>MADKLFINALKKKFEESPEEKKTTFYTLGGWKQSERKTEFVNAGKEVAAKRGIPQYNPDIGTPLGQRVLMPYQVSTTDTYVEGDDLHFVNNAAMQQMWDDIRRTVIVGLNHAHAVIEKRLGKEVTPETITHYLETVNHAMPGAAVVQEHMVETHPALVADSYVKVFTGNDEIADEIDPAFVIDINKQFPEDQAETLKAEVGDGIWQVVRIPTIVSRTCDGATTSRWSAMQIGMSMISAYKQAAGEAATGDFAYAAKHAEVIHMGTYLPVRRARGENEPGGVPFGYLADICQSSRVNYEDPVRVSLDVVATGAMLYDQIWLGSYMSGGVGFTQYATAAYTDNILDDFTYFGKEYVEDKYGLCEAPNNMDTVLDVATEVTFYGLEQYEEYPALLEDQFGGSQRAAVVAAAAGCSTAFATGNAQTGLSGWYLSMYLHKEQHSRLGFYGYDLQDQCGASNVFSIRGDEGLPLELRGPNYPNYAMNVGHQGEYAGISQAPHAARGDAFVFNPLVKIAFADDNLVFDFTNVRGEFAKGALREFEPAGERALITPAK[2x];>MAKFEDKVDLYDDRGNLVEEQVPLEALSPLRNPAIKSIVQGIKRTVAVNLEGIENALKTAKVGGPACKIMGRELDLDIVGNAESIAAAAKEMIQVTEDDDTNVELLGGGKRALVQVPSARFDVAAEYSAAPLVTATAFVQAIINEFDVSMYDANMVKAAVLGRYPQSVEYMGANIATMLDIPQKLEGPGYALRNIMVNHVVAATLKNTLQAAALSTILEQTAMFEMGDAVGAFERMHLLGLAYQGMNADNLVFDLVKANGKEGTVGSVIADLVERALEDGVIKVEKELTDYKVYGTDDLAMWNAYAAAGLMAATMVNQGAARAAQGVSSTLLYYNDLIEFETGLPSVDFGKVEGTAVGFSFFSHSIYGGGGPGIFNGNHIVTRHSKGFAIPCVAAAMALDAGTQMFSPEATSGLIKEVFSQVDEFREPLKYVVEAAAEIKNEI[2x];>[2x]MAQYYPGTTKVAQNRRNFCNPEYELEKLREISDEDVVKILGHRAPGEEYPSVHPPLEEMDEPEDAIREMVEPIDGAKAGDR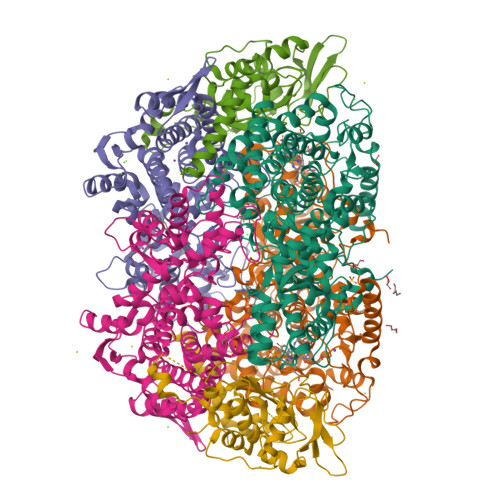VRYIQFTDSMYFAPAQPYVRSRAYLCRYRGADAGTLSGRQIIETRERDLEKISKELLETEFFDPARSGVRGKSVHGHSLRLDEDGMMFDMLRRQIYNKDTGRVEMVKNQIGDELDEPVDLGEPLDEETLMEKTTIYRVDGEAYRDDVEAVEIMQRIHVLRSQGGFNLE> GSGSGSGSGSSKFSNITIKNFRNFEKVNINLDNKNVIFGMNDIGKTNFLYALRFLLDKEIRKFGFNKSDYHKHDTSKKIEIILTLDLSNYEKDEDTKKLISVVKGARTSANADVFYIALESKYDDKELYGNIILKWGSELDNLIDIPGRGNINALDNVFKVIYINPLVDLDKLFAQNKKYIFEESQGNESDEGILNNIKSLTDQVNQQIGEMTIIKGFQQEITSEYRSLKKEEVSIELKSEMAIKGFFSDIIPYIKKDGDSNYYPTSGDGRRKMLSYSIYNYLAKKKYEDKIVIYLIEEPEISLHRSMQIALSKQLFEQSTYKYFFLSTHSPELLYEMDNTRLIRVHSTEKVVCSSHMYNVEEAYGSVKKKLNKALSSALFAERVLLIEGPSEKILFEKVLDEVEPEYELNGGFLLEVGGTYFNHYVCTLNDLGITHIIKTDNDLKSKKGKKGVYELLGLNRCLNLLGRENLDEITIDIPEDIKGKKKKERLNERKKEIFKQYKNEVGEFLGERIYLSEIDLENDLYSAIGESMKRIFENEDPVHYLQKSKLFNMVELVNNLSTKDCFDVFEHEKFACLKELVGSDRG;> SREQIIKDGGNILVTAGAGSGKTTILVSKIEADLKENKTHYSIAAVTFTNKAAKEIEGRLGYSSRGNFIGTNDGFVESEIIRPFIKDAFGNDYPDNFTA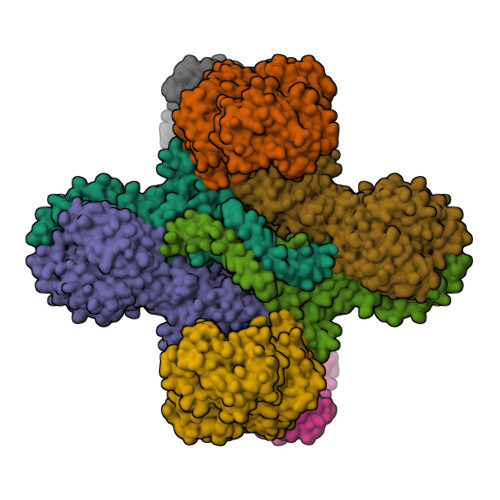EYFDNQFASYDKGLQVLKYQNILGTYSNPKKNFKFQLALDILKKSLVARQYIFSKYFKIFIDEYQDSDKDMHNLFMYLKDQLKIKLFIVGDPKQSIYIWRGAEPENFNGLIENSTDFNKYHLTSNFRCCQDIQNYSNLFNEETRSLIKEKNEVQNVISIADDMPISDILLKLTEEKQVLNIEAELVILVRRRNQAIEIMKELNEEGFNFIFIPQTPLDRATPNATLLKEVIKYVKNDRYSIYDLAAEIVGNLSSREIKEIQKIINELLVPNINQVLINQVLINLFAKLEITLDTREITAFTEVMMTNEFDIAFDTNEYLHKIFTVHSAKGLEFNQVIITASDYNVHYNRDTNEHYVATTRAKDKLIVIMDNKKYSDYIETLMKELKIKNIIKSI> AA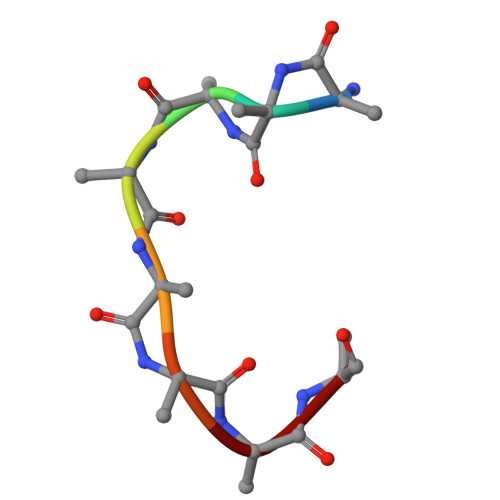AAAAAA> HHHHMPVFHTRTIESILEPVAQQISHLVIMHEEGEVDGKAIPDLTAPVAAVQAAVSNLVRVGKETVQTTEDQILKRDMPPAFIKVENACTKLVQAAQMLQSDPYSVPARDYLIDGSRGILSGTSDLLLTFDEAEVRKIIRVCKGILEYLTVAEVVETMEDLVTYTKNLGPGMTKMAKMIDERQQELTHQEHRVMLVNSMNTVKELLPVLISAMKIFVTTKNSKNQGIEEALKNRNFTVEKMSAEINE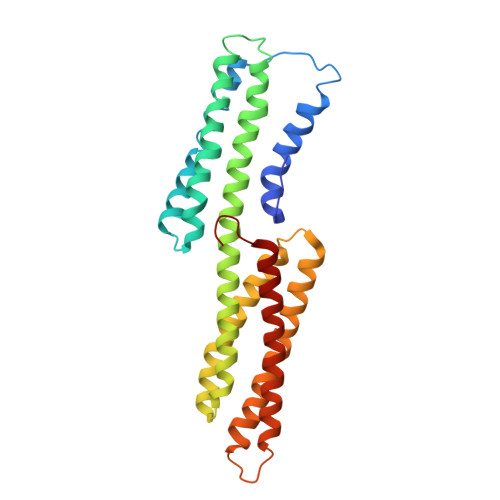IIRVLQLTSWDEDAW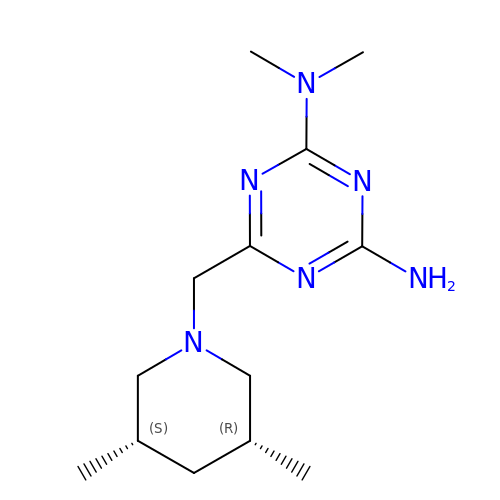6-{[(3R,5S)-3,5-dimethylpiperidin-1-yl]methyl}-N,N-dimethyl-1,3,5-triazine-2,4-diamine | C13 H24 N6 | XCUJQKCZUHQRMB-AOOOYVTPSA-N> SMQFSKMHGLGNDFMVVDAVTQNVFFSPELIRRLADAHLGVGFDQLLVVEPPYDPELDFHYRIFNADGSEVAQCGNGARCFARFVRLKGLTNKRDIRVSTANGRMVLTVTDDDLVRVNMGEPNFEPSAVPFRANKAEKTYIMRAAEQTILCGVVSMGNPHCVIQVDDVDTAAVETLGPVLESHERFPERANIGFMQVVKREHIRLRVYERGAGETQACGSGACAAVAVGIQQGLLAEEVRVELPGGRLDIAWKGPGHPLYMTGPAVHVADGFIHL;> SMIDDDGYRPNVGIVICNRQGQVMWARRFGQHSWQFPQGGINPGESAEQAMYRELFEEVGLSRKDVRILASTRNWLRYKLPKRLVRWDTKPVCIGQKQKWFLLQLVSGDAEINMQTSSTPEFDGWRWVSYWYPVRQVVSFKRDVYRRVMKEFASVVMSLAA

Finding a correct substrate is especially difficult for the Escherichia coli Nudix hydrolase RppH, which triggers 5′-end-dependent RNA degradation by removing orthophosphate from the 5′-diphosphorylated transcripts. In Escherichia coli and probably many other bacteria, RppH converts diphosphorylated 5′ ends of transcripts into monophosphorylated ends that accelerate subsequent cleavage by the 5′-monophosphate-stimulated endonuclease RNase E. Escherichia coli RppH can also remove pyrophosphate from triphosphorylated RNA with lower efficiency. Here we show that RppH binds and slowly hydrolyzes NTPs, NDPs and (p)ppGpp, which each resemble the 5′-end of RNA. A series of X-ray crystal structures of RppH-nucleotide complexes, trapped in conformations either compatible or incompatible with hydrolysis, explain the low reaction rates of mononucleotides and suggest two distinct mechanisms for their hydrolysis.

GDP is too small for its terminal phosphate to reach even an extended catalytic site if its nucleobase binds to RppH in the same way as GTP. Instead, the structure of RppH bound to GDP and Mg2+, determined at 2.7 Å resolution, revealed that GDP slides toward the catalytic site by a distance that roughly corresponds to two phosphates of GTP. As a result, the 5′ α-phosphate of GDP occupies the position of the 5′ γ-phosphate of GTP and maintains two of the corresponding intermolecular contacts with RppH. The β-phosphate of GDP moves deeper into the active site, where it replaces Mg4. Therefore, the catalytic site in the GDP-bound structure contains three Mg2+ cations in a configuration remarkably similar to that observed in the RNA-bound structure. RppH likely catalyzes cleavage between the two phosphates of GDP by using a nucleophilic water molecule or hydroxide ion positioned between Mg2 and Mg3, as proposed for RNA substrates. In the crystal structure, this nucleophile is replaced by a fluoride ion located a short distance (3.2 Å) from the β-phosphorus atom, at a 157° angle compatible with in-line attack. In contrast to the second nucleobase of RNA, which inserts deeply into the protein cleft, insertion of the nucleobase of GDP is shallower and lacks some contacts formed by RppH-bound RNA. In particular, the GDP-Mg2+-F−-RppH structure shows the nucleobase of mononucleotide substrates emerging from the deep cleft and moving toward the catalytic site, causing it to lose some interactions with the protein but enabling the 5′-terminal phosphates to reach the catalytic site. With GDP bound in this manner, a nucleophile is well situated for in-line attack on the β-phosphorus atom.>MKIFLDTANIDEIRTGVNWGIVDGVTTNPTLISKEAVNGKKYGDIIREILKIVDGPVSVQVVSTKYEGMVEEARK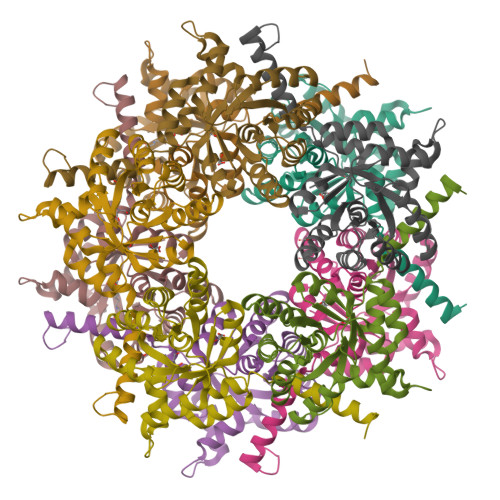IHGLGDNAVVKIPMTEDGLRAIKTLSSEHINTNCTLVFNPIQALLAAKAGVTYVSPYVGRLDDIGEDGMQIIDMIRTIFNNYIIKTQILVASIRNPIHVLRSAVIGADVVTVPFNVLKSLMKHPKTDEGLAKFLEDWKKVSPDGKLIL[5x]>MKKGHHHH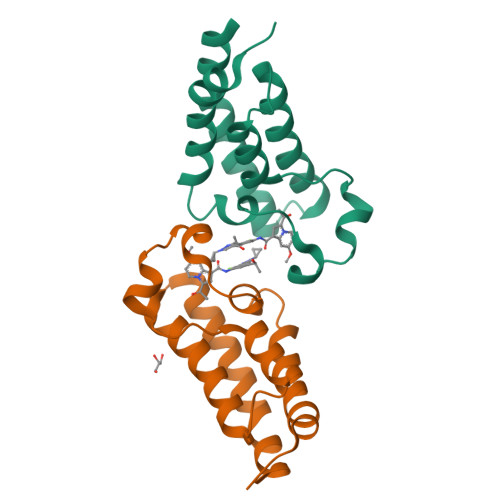HHLVPRGSRKKIFKPEELRQALMPTLEALYRQDPESLPFRQPVDPQLLGIPDYFDIVKNPMDLSTIKRKLDTGQYQEPWQYVDDVWLMFNNAWLYNRKTSRVYKFCSKLAEVFEQEIDPVMQSLG[2x]>[2x]MSIKIRDFGLGSDLISLTNKAGVTISFTNLGARIVDWQKDGKHLILGFDSAKEYLEKDAYPGATVGPTAGRIKDGLVKISGKDYILNQNEGPQTLHGGEESIHTKLWTYEVTDLGAEVQVKFSLVSNDGTNGYPGKIEMSVTHSFDDDNKWKIHYEAISDKDTV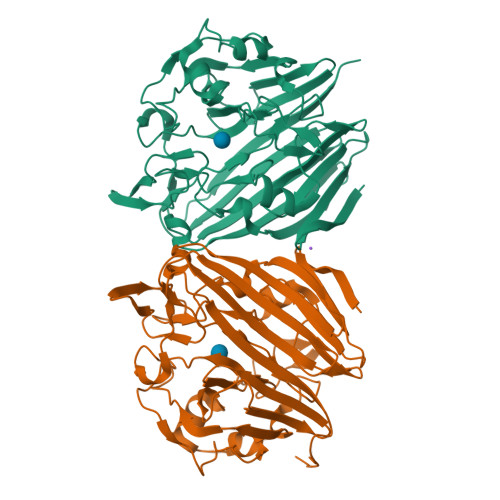FNPTGHVYFNLNGDASESVENHGLRLAASRFVPLKDQTEIVRGDIVDIKNTDLDFRQEKQLSNAFNSNMEQVQLVKGIDHPFLLDQLGLDKEQARLTLDDTSISVFTDQPSIVIFTANFGDLGTLYHEKKQVHHGGITFQCQVSPGSEQIPELGDISLKAGEKYQATTIYSLHTKLEHHHHHH5-AMIDINO-BENZIMIDAZOLE | C8 H9 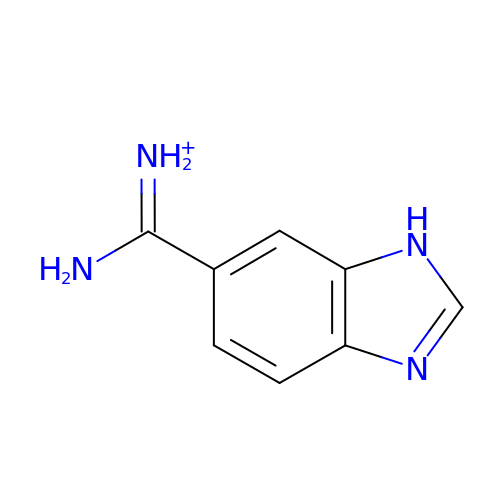N4 | UHGFPMUGEQINGV-UHFFFAOYSA-O> GTKQRADIVMSEAEIADFVNSSRTGTLATIGPDGQPHLTAMW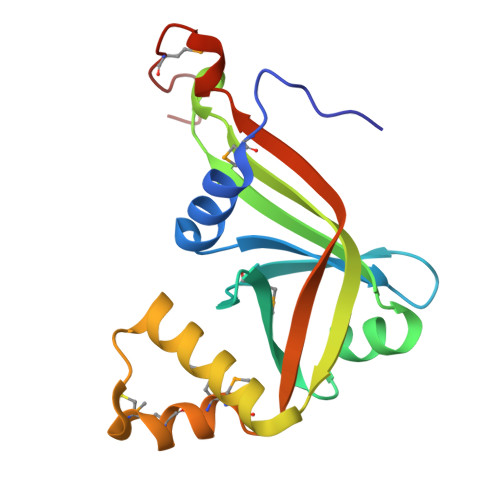YAVIDGEIWLETKAKSQKAVNLRRDPRVSFLLEDGDTYDTLRGVSFEGVAEIVEEPEALHRVGVSVWERYTGPYTDECKPMVDQMMNKRVGVRIVARRTRSWDHRKLGLPHMSVGGSTAP> TRFTEEYQLFEELGKGAFSVVR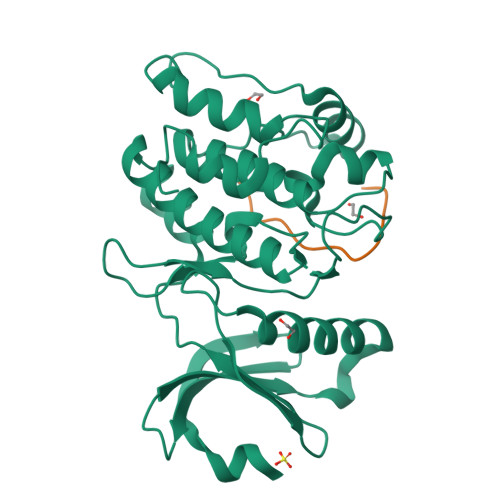RCVKVLAGQEYAAKIINTKKLSARDHQKLEREARICRLLKHPNIVRLHDSISEEGHHYLIFDLVTGGELFEDIVAREYYSEADASHCIQQILEAVLHCHQMGVVHRDLKPENLLLASKLKGAAVKLADFGLAIEVEGEQQAWFGFAGTPGYLSPEVLRKDPYGKPVDLWACGVILYILLVGYPPFWDEDQHRLYKQIKAGAYDFPSPEWDTVTPEAKDLINKMLTINPSKRITAAEALKHPWISHR;> KAQKKNRNKLRRQHSYDTFVDL>[2x]SDRPLSVHLNLGQKGNRKTSCPIKINQFEGHFMKLQADSNYLLSKEYEELKDVGRNQSCDIALLPENRGKNRYNNILPYDATRVKLSNVDDDPCSDYINASYIPGNNFRREYIVTQGPLPGTKDDFWKMVWEQNVH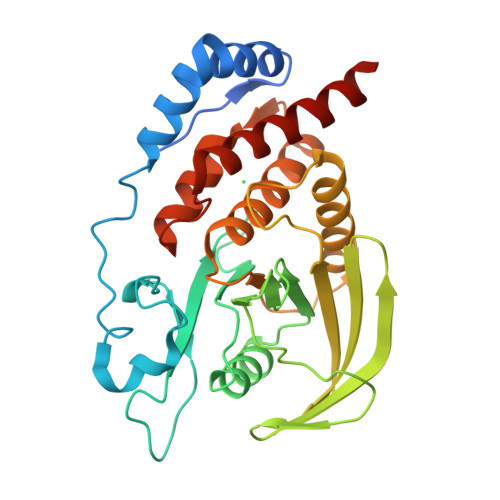NIVMVTQCVEKGRVKCDHYWPADQDSLYYGDLILQMLSESVLPEWTIREFKICGEEQLDAHRLIRHFHYTVWPDHGVPETTQSLIQFVRTVRDYINRSPGAGPTVVHCSAGVGRTGTFIALDRILQQLDSKDSVDIYGAVHDLRLHRVHMVQTECQYVYLHQCVRDVLRARKLRSEQ> MSRKRSTKPKPAAKIALKKENDQFLEALKLYEGKQYKKSLKLLDAILKKDGSHVDSLALKGLDLYSVGEKDDAASYVANAIRKIEGASASPICCHVLGIYMRNTKEYKESIKWFTAALNNGSTNKQIYRDLATLQSQIGDFKNALVSRKKYWEAFLGYRANWTSLAVAQDVNGERQQAINTLSQFEKLAEGKISDSEKYEHSECLMYKNDIMYKAASDNQDKLQNVLKHLNDIEPCVFDKFGLLERKATIYMKLGQLKDASIVYRTLIKRNPDNFKYYKLLEVSLGIQGDNKLKKALYGKLEQFYPRCEPPKFIPLTFLQDKEELSKKLREYVLPQLERGVPATFSNVKPLYQRRKSKVSPLLEKIVLDYLSGLDPTQDPIPFIWTNYYLSQHFLFLKDFPKAQEYIDAALDHTPTLVEFYILKARILKHLGLMDTAAGILEEGRQLDLQDRFINCKTVKYFLRANNIDKAVEVASLFTKNDDSVNGIKDLHLVEASWFIVEQAEAYYRLYLDRKKKLDDLASLKKEVESDKSEQIANDIKENQWLVRKYKGLALKRFNAIPKFYKQFEDDQLDFHSYCMRKGTPRAYLEMLEWGKALYTKPMYVRAMKEASKLYFQMHDDRLKRKSDSLDENSDEIQNNGQNSSSQKKKAKKEAAAMNKRKETEAKSVAAYPSDQDNDVFGEKLIETSTPMEDFATEFYNNYSMQVREDERDYI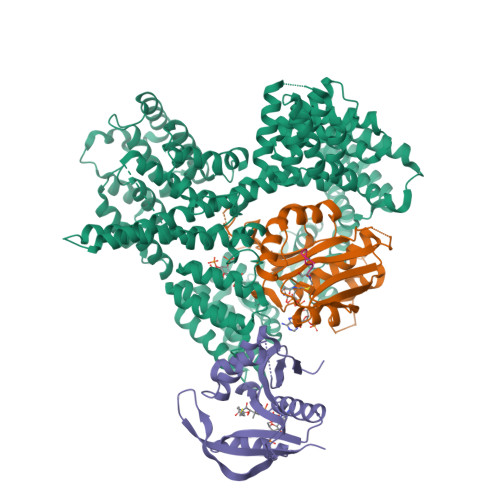LDFEFNYRIGKLALCFASLNKFAKRFGTTSGLFGSMAIVLLHATRNDTPFDPILKKVVTKSLEKEYSENFPLNEISNNSFDWLNFYQEKFGKNDINGLLFLYRYRDDVPIGSSNLKEMIISSLSPLEPHSQNEILQYYL;> MPINIRRATINDIICMQNANLHNLPENYMMKYYMYHILSWPEASFVATTTTLDCEDSDEQDENDKLELTLDGTNDGRTIKLDPTYLAPGEKLVGYVLVKMNDDPDQQNEPPNGHITSLSVMRTYRRMGIAENLMRQALFALREVHQAEYVSLHVRQSNRAALHLYRDTLAFEVLSIEKSYYQDGEDAYAMKKVLKLEELQISNFTHRRLKENEEKLEDDLESDLLEDIIKQGVNDIIV;> MGRDICTLDNVYANNLGMLTKLAHVTVPNLYQDAFFSALFAEDSLVAKNKKPSSKKDVHFTQMAYYSEIPVGGLVAKLVPKKQNELSLKGIQIEFLGVLPNYRHKSIGSKLLKFAEDKCSECHQHNVFVYLPAVDDLTKQWFIAHGFEQVGETVNNFIKGVNGDEQDAILLKKHIS;> SYSMEHFR> AEGDTLISVDYEIFGKVQGVFFRKYTQAEGKKLGLVGWVQNTDQGTVQGQLQGPASKVRHM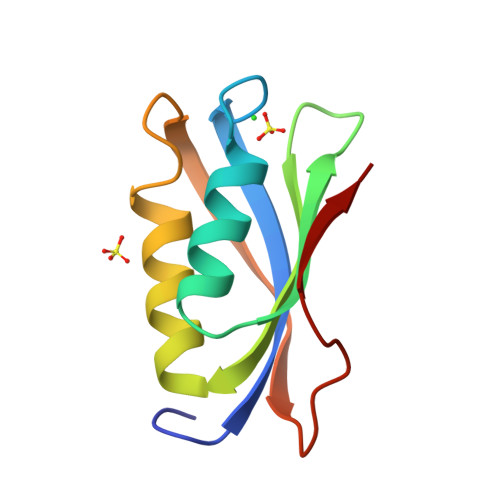QEWLETKGSPKSHIDRASFHNEKVIVKLDYTDFQIVK> MGRVADTIARGPSNSEQIPALTAVETGHTSQVDPSDTMQTRHVHNYHSRSESSIENFLCRSACVIYIKYSSAESNNLKRYAEWVINTRQVAQLRRKMEMFTYIRCDMELTFVITSHQEMSTATNSDVPVQTHQIMYVPPGGPVPTSVNDYVWQTSTNPSIFWTEGNAPPRMSIPFMSIGNAYTMFYDGWSNFSRDGIYGYNSLNNMGTIYARHVNDSSPGGL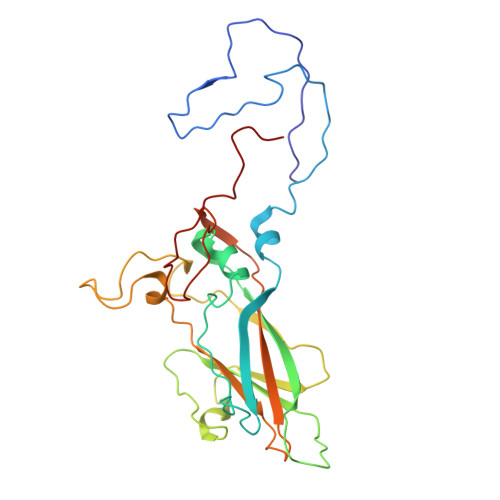TSTIRIYFKPKHVKAYVPRPPRLCQYKKAKNVNFDVEAVTTERASLVTT> MASHLASIYGTEQDKVNCSFYYKIGACRHGERCSRKHVKPNFSQTILCPNMYKNPIHEPNGKKFTQRELAEQFDAFYEDMFCEFSKYGEVEQLVVCDNVGDHLVGNVYVRFKYEESAQNAIDDLNSRWYSQRPVYAELSPVTDFREACCRQHETSECQRGGLCNFMHAKKPSPQLLRDLVLAQRKYLALNAAEEMKKEPNSDSTNRWVSVTAERK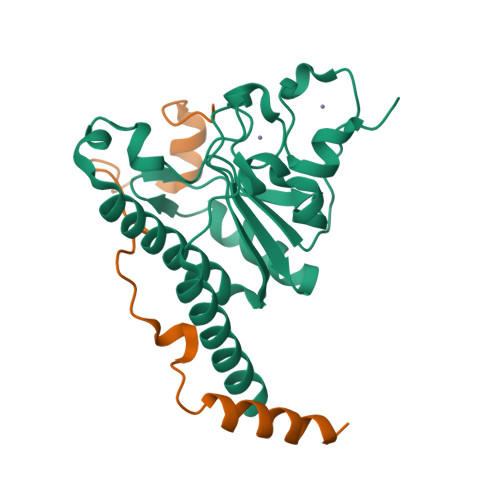N;> GGSSVGRSRSPPPSRERSVRSIEQELEQLRDVTPINQWKRKRSLWDIKPPGYELVTADQAKMSGVFPLPGA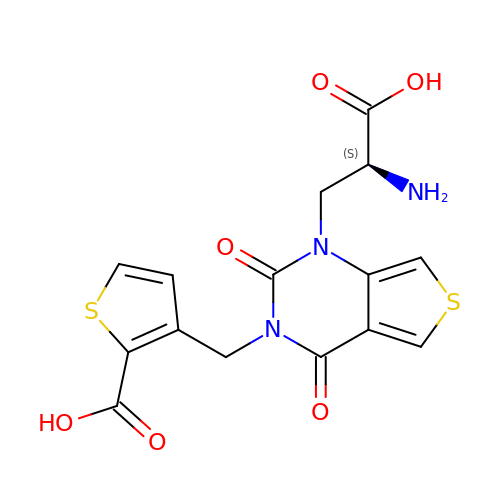(S)-1-(2'-AMINO-2'-CARBOXYETHYL)-3-[(2-CARBOXYTHIEN-3-YL)METHYL]THIENO[3,4-D]PYRIMIDIN-2,4-DIONE | C15 H13 N3 O6 S2 | LSNSPQPOGKSTHQ-VIFPVBQESA-N> GEPEVTDQLEWQSNQPWEQALNRFWDYLRWVQ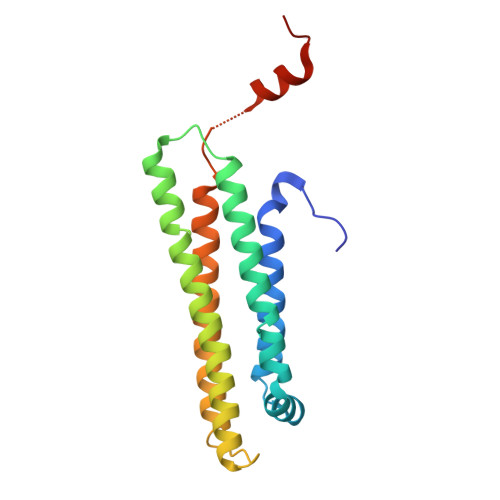TLSDQVQEELQSSQVTQELTALMEDTMTEVKAYKKELEEQLGPVAEETRARLGKEVQAAQARLGADMEDLRNRLGQYRNEVHTMLGQSTEEIRARLSTHLRKMRKRLMRDAEDLQKRLAVYKAGAREGAERGVSAIRERLGPLVEQGRQ> MGGGLPPKRSEVAESQPASSASSSAAAPAPAAETAGPKLPPRPAGLGLGGAGLLPSRGAAAAPSAGSATGTPAAAASSSLQQQQQQPAPPATQPAAHAAPAAPAGLGGAGLKPMLPPRPAAAAGAGAAGAAAAKPTPAPAPAAAPVPAAAPPPRPAMPNPAAGMSLPPRPVVAAAPPVLAAAGSDAVVDPSEDRRVQRVQRIAHDTRVRLIRAASRLGLAPRTDQVAQFLQAIERSERMVGAQHYKGSRRVDLLAAAEREARLAEEREGAAAEAVAGLRVKILVLGMTGTGKTELINSLLNRPAGSRTNAFREATRRVRVVRGDHNGIPLTFIDTPGLHASASRTADNRAILRAVRAAYRWHKPDYVFYVDRLDATRPGFGEMGLLGLITESLGAGVWRNTMAVLTHAHAARTA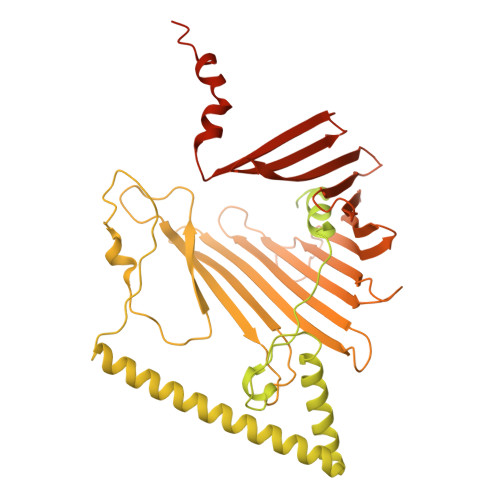FGGQYDVNSRQRRNIVSQLLRQAAGDQQSRNPVFLADCHPACPTNSLGQPVILEGPTAVPWKQQLLVQLVGYKSYNVATSAFKDLAKAKAGKAAAGAAGGARGPQDIFKQMMRSRLPPMTFFVEQMSEGVLKPEGWATMETVAGLGEEVTEDEGAESFNHVYYRQMYELAVAGDPWAQREYAAMLRAYDKGCESYRASYEEADVDANVEYGVESYVVDPIDFGPSFDPEDMYSHRHAYAEAADAGVTVIPSQDYYGPEHDDPLNGIVFQYEAQPFSRHGWGGVPFDLTVCCEKDKTSLCLQGETHVSLVHSVPPFGPRHITQVTGSWEVLRPNIKDVMYQLEVDTFKDGLLGKSDHAGCGLMLARLGEGGDPRKGPTAVGVRLQDTLRVGPFKLEACASKVAVQGPTGGKEEGWGARAFVGYDWLPGLGMAFDFIQERTPEEGGKRLRGYGANFTYDWEALGAAFGMEVDYVAASESVFVSVNAFSGNDYRLGWLLLLPAVNYFKETVSSLWARLRGAGGGEGEEGEELEEEGEGEEGDDEEAMMMMAQEGDL> AIWRSRSFDEAIEMFRESLYSAKNEVIVVTPSEFFETIREDLIKTLERGVTVSLYIDKIPDLSEFKGKGNFFVRQFYKLNHLIGMTDGKEVVTIQNATFDSIGPPSFKSTYPEIIF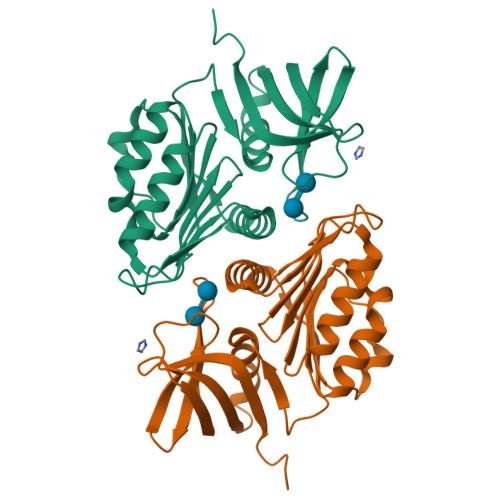SQYSLIIEIFKESTLEKEIIGNPKDIRFFAMFHAVDFVKNHLKNRNIYAEITGKNLESGRLETLTGRVVGYTLSLREAVNNIHLETENGVVKVGGMFAVIEDYESTEIKFIMGGSRS>MADRAKLLTTPGVFGNFSTYKVRADYMKLPAAERKAAAAEAQMVIDKHKDKVIVDTYLTRGLGAGSDYLLRVHSTDMAATQAFLVDWRATKLGMYSDVTENLVGITKALNYISKDKSPDLNAGLSSATYSDSAPRYVIVIPVKKDAAWWNMSDEQRLKEIEVHTQPTLQYLVNVKRKLY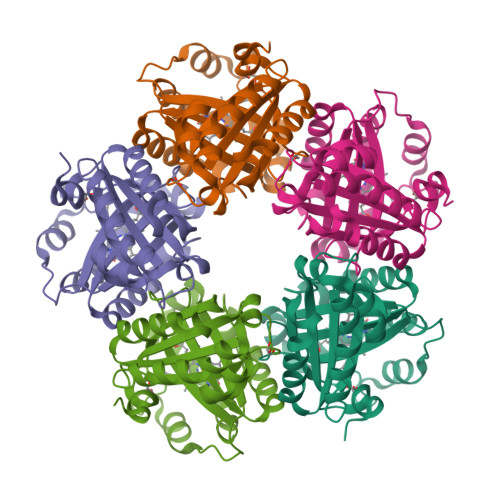HSTGLADADFITYFETADLAAFNNLLIALAKVPENTHHVRWGNPTVLGTIQSADVLVKTLSGM[5x]>SMRKSREYEHVRRDLDPNEVWEIVGELGDGAFGKVYKAKNKETGALAAAKVIETKSEEELEDYIVEIEILATCDHPYIVKLLGAYYHDGKLWIMIEFCPGGAVDAIMLELDRGLTEPQIQVVCRQMLEALNFLHSKRIIHRDLKAGNVLMTLEGDIRLADFGVSAKNLKTLQKRDSFIGTPYWMAPEVVMCETMKDTPYDYKADIWSLGITLIEMAQIEPPHHELNPMRVLLKIAKSDPPTLLTPSKWSVEFRDFLKIALDKNPETRPSAAQLLEHPFVSSITSNKALRELVA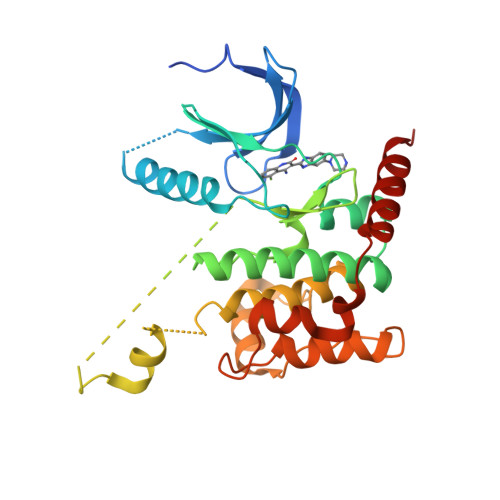EAKAEVMEE[2x]>[3x]MGSSHHHHHHSSGRENLYFQGMESVNTSFLSPSLVTIRDFDNGQFAVLRIGRTGFPADKGDIDLCLDKMKGVRDAQQSIGDDTEFGFKGPHIRIRCVDIDDKHTYNAMVY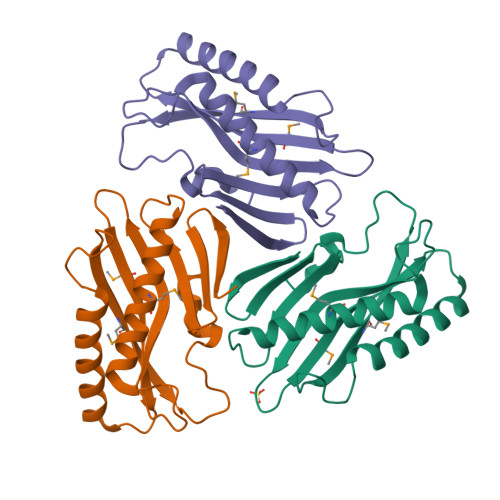VDLIVGTGASEVERETAEELAKEKLRAALQVDIADEHSCVTQFEMKLREELLSSDSFHPDKDEYYKDFL> GKELEIVARLQQLNIELARKLLEAVARLQELNIDLVRKTSELTDEKTIREEIRKVKEESKRIVEEAEQEIRKAEAESLRLTAEAAADAARKAALRMGDERVRRLAAELVRLAQEAAEEATRDPNSSDQNEALRLIILAIEAAVRALDKAIEKGDPEDRERAREMVRAAVRAAELVQRYPS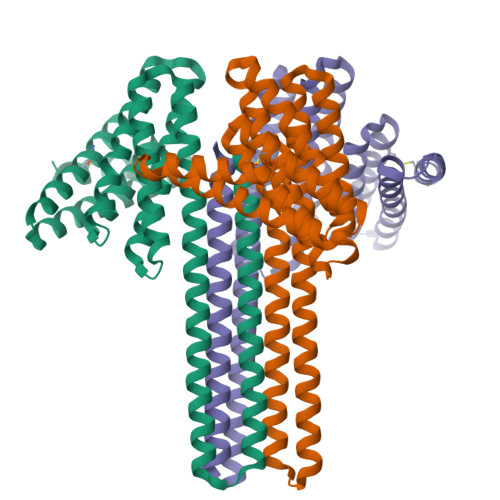ASAANEALKALVAAIDEGDKDAARCAEELVEQAEEALRKKNPEEARAVYEAARDVLEALQRLEEAKRRGDEEERREAEERLRQACERARKKN> GPLGSMTGAATAA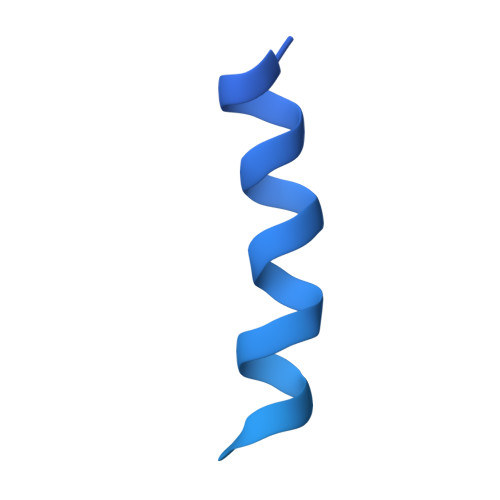ENSATQLEFYRKALNFNVIGRYDPKIKQLLFHTPHASLYKWDFKKDEWNKLEYQGVLAIYLRDVSQNTNLLPVSPQEVDIFDSQNGSNNIQVNNGSDNSNRNSSGNGNSYKSNDSLTYNCGKTLSGKDIYNYGLIILNRINPDNFSMGIVPNSVVNKRKVFNAEEDTLNPLECMGVEVKDELVIIKNLKHEVYGIWIHTVSDRQNIYELIKYLLENEPKDSFA>HHHHHHHHGSSLEVLFQGPA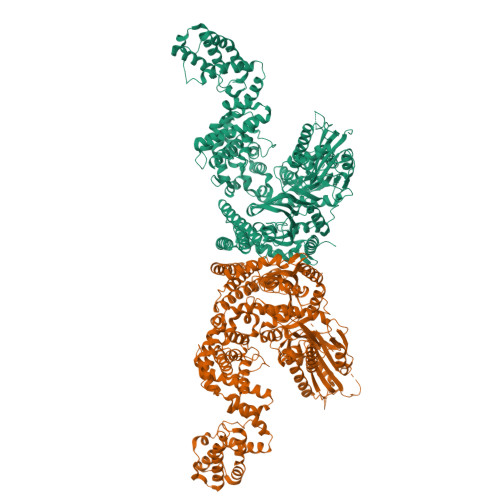VASADGDAPSPVSVSASAATKGPSSSSVLTFQQAIQRLQDYWASVGCAVMQCSNTEVGAGTMNPLTFLRVLGPEPWNVAYVEPSIRPDDSRYGDNPNRLQRHTQFQVILKPDPGNSQDLFLHSLSALGINVREHDIRFVEDNWESPVLGAWGLGWEVWMDGMEITQFTYFQQSGSLPLLPVSVEITYGLERILMSLQGVDHFKNIQYTKGITYGELFLENEKEMSAYYLEHANVDNIQKHFDDFEEEARSLLSLWLPIPAYDHVLKASHAFNILDSRGFVGVTERARYFGRMRSLARQCAQLWVKTRENLGYPLGTYQESNLIYPHVSEKPSRKGVVGQPRAFVLEIGTEELPPHDVIEATKQLEKSLIQILEKRRLSHGKVRSYGTPRRLAVVVENLNMKQMEEEIELRGPPVAKAFDQEGRPTKAAEGFCRKNNVPIDSLYRRTDGKTEYIYARVKESARFADEVLTEDLPTIISGISFPKSMRWNSNIVFSRPIRWIFALHGDLIVPFCFAGISSGNQSCGLRNSSLANFKVEAAELYLHTLEKAGILIDMQERKQRILHDSSILAEGVGGDIIAPDSLVQEVINLVEAPMPIIGRYDVSFLALPKDVLITVMQKHQKYFPVTSKTMGNLLPCFITVANGAIKEEVVRKGNEAVLRARYEDAKFFYKMDTQKKLSEFRDQLSSILFHERLGTMLDKMKRVENTVAEVALLLGINEKMIPAIKDAAALAMSDLATNIVTEFTSLAGIMARHYALRDGLSEQIAEALFEITLPRFSGDVFPKTDPGIVLAVTDRLDSLVGLFGAGCQPSSTNDPFGLRRISYGLVQILVENKKNFDLTKALTLVAEEQPITIDSGVIDEVVQFVTRRLEQLLVDEGINCEIVRSVLIERANCPYLASQTAIEMEAFSRTEDFPKIVEAYSRPTRIIRGKEIGSALEVDASVFEKDEERALWSAYLEVADKIHPGVDIKAFADASLELLQPLEDFFTNVFVMAEDEKVRNNRLALLTKVASLPKGIADLSVLPGF[2x]> MARSVSSLQSLCITKISENISKWQKEADESSKLVFNKLRDVLGGVSTANLNNLAKALSKNRALNDHTLQLFLKTDLKRLTFSDCSKISFDGYKTLAIFSPHLTELSLQMCGQLNHESLLYIAEKLPNLKSLNLDGPFLINEDTWEKFFVIMKGRLEEFHISNTHRFTDKSLSNLLINCGSTLVSLGLSRLDSISNYALLPQYLVNDEFHSLCIEYPFNEEDVNDEIIINLLGQIGRTLRKLVLN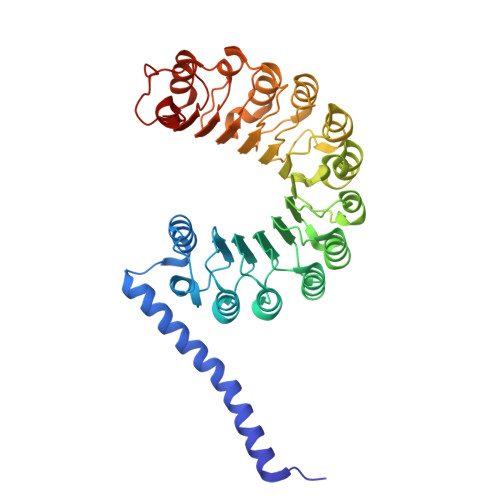GCIDLTDSMIINGLTAFIPEKCPLEVLSLEESDQITTDSLSYFFSKVELNNLIECSFRRCLQLGDMAIIELLLNGARDSLRSLNLNSLKELTKEAFVALACPNLTYLDLGFVRCVDDSVIQMLGEQNPNLTVIDVFGDNLVTEKATMRPGLTLIGRQSDSI1-(4-{3,5-dichloro-4-[(2-methylpyridin-3-yl)methoxy]phenyl}pyridin-2-yl)piperazine | C22 H22 Cl2 N4 O | 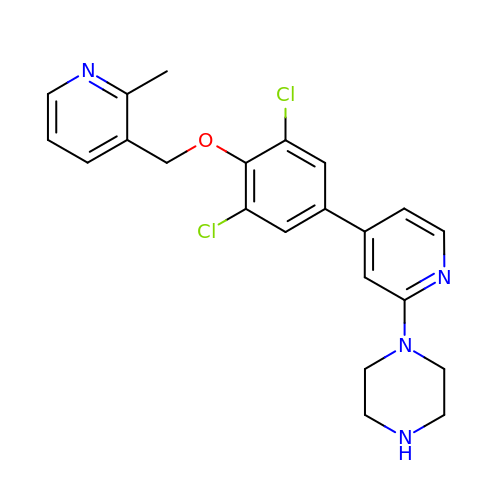KDTZTRFMUYKFDT-UHFFFAOYSA-N> GVKTFQFPFAEQLEKVAEQFPTFQILNEEGEVVNEEAMPELSDEQLKELMRRMVYTRILDQRSISLNRQGRLGFYAPTAGQEASQIASHFALEKEDFILPGYRDVPQIIWHGLPLYQAFLFSRGHFHGNQIPEGVNVLPPQIIIGAQYIQAAGVALGLKMRGKKAVAITYTGDGGTSQGDFYEGINFAGAFKAPAIFVVQNNRFAISTPVEKQTVAKTLAQKAVAAGIPGIQVDGMDPLAVYAAVKAARERAINGEGPTLIETLCFRYGPHTMSGDDPTRYRSKELENEWAKKDPLVRFRKFLEAKGLWSEEEENNVIEQAKEEIKEAIKKAD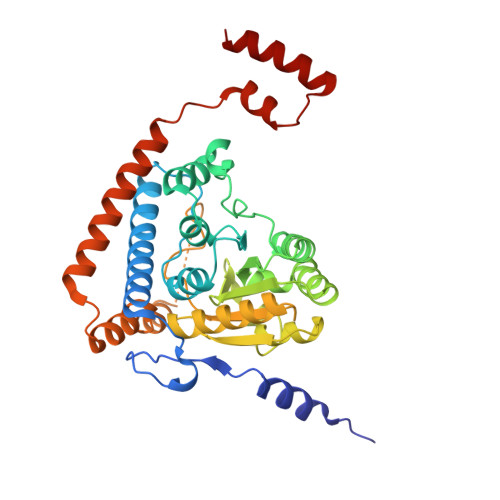ETPKQKVTDLISIMFEELPFNLKEQYEIYKEKESK> MTFTQTNDPTIRKYVQSWQKLDVDEQLALFWFIYKEMGGAITPAA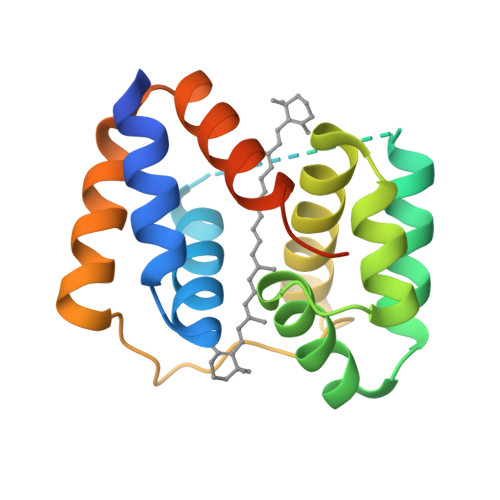PGASTVSPAIAEGLFNQVKELNHEQQLQLQRDLIRRVDNQLSREYGSLGDTTKLLFWYLLSQGMDNATIVPFPADYKLSSESQELLEGIKGLGFEQQITLFRDYVSPMGAEAKAGAEIHHHHHH>SNAADALADMCARLEAGSGGRLGV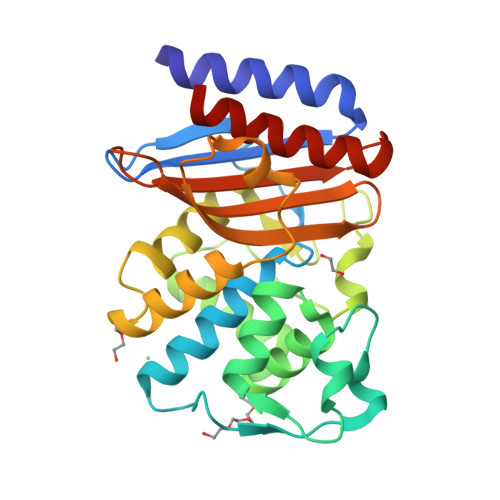GVLDTASGRMIGHRLDDRFPMCSTFKVLAAGLVLARVDRKQENLDRRVSYAKSDLVTYSPATEKHVEDGMTIAELCEAAITLSDNTAANLLLASFGGPAGLTAFARSLGDETTRLDRIETELNEALAGDPRDTTSPRAMAQDLRALTLGDALSPASRAQLITWLKANTTGGTRLRAGVPPGWTVGDKTGTGGRGTANDIAVLWPLQRAPLIVTVYLTGATVVRDQQNKIIADVGAAVAGAMHG[2x]> MTSVEELYVINPINQWPAPGSFSSQKPPGTLLPGEDPEAVFKQYHVVYLVPGAQYHWKNILIEKPVWIYGNGATVRTSGTGPILRIVGNRTEKRDVRIQDISFFGEDCTPNRMEPMSEKLVYQMAIWVTDMKRVTIKGCNFTNFAGAAVFFEETAYNGFFWSMQHLITECRFTGCRIGIANGGRSEYSTASFNNFFDCQICFNVVGGNWNRCGNIAANCRCVYLHTTNMWYEGAGGNFNAAHGSFTGNTMNHCDYGGNLWPTAFQLPDREIQL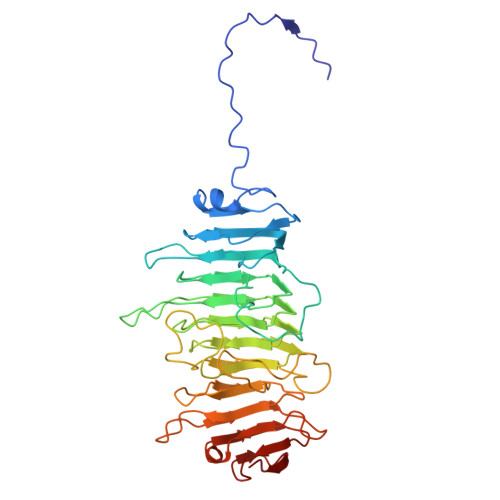AGFYFDNARARCPTWTGNTQYYGDMKILNFNQANDAAIFVIDGCALYGQPGDTGSIETTAALTDKVFIQGCQGNKVTLFNIKAANVVPAIGTIKQKP>[2x]GHMNDALHIGLPPFLVQANNEPRVLAAPEARMGYVLELV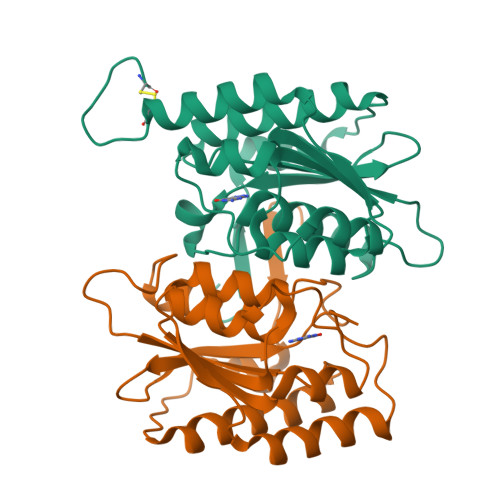RANIAADGGPFAAAVFERDSGLLIAAGTNRVVPGRCSAAHAEILALSLAQAKLDTHDLSADGLPACELVTSAEPCVMCFGAVIWSGVRSLVCAARSDDVEAIGFDEGPRPENWMGGLEARGITVTTGLLRDAACALLREYNACNGVIYNARCGVHKGS>GAMDPEFSAQLGAMQHLKDQLEQRTRMIEANIHRQQEELRKIQEQLQMVHG[4x];>[2x]GNTLVVLHKSGLL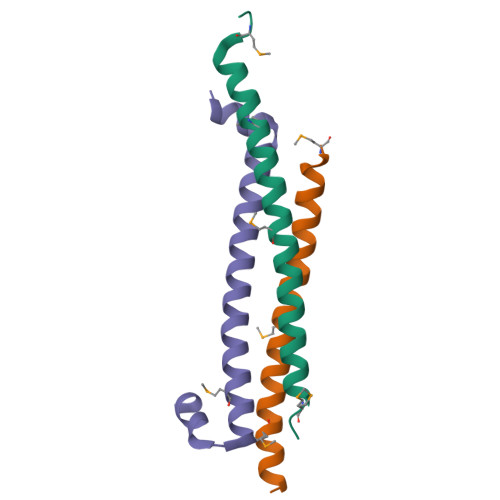EITLKTKELIRQNQATQAELDQLKEQTQMFIEATKSRAPQAWAKLQASLTS> DADKLPHTKVTLVAPPQVHPHEQATKSGPKVVEFTMTIEEKKMVIDDKGTTLQAMTFNGSMPGPTLVVHEGDYVQLTLVNPATNAMPHNVDFHGATGALGGAKLTNVNPGEQATLRFKADRSGTFVYHCAPEGMVPWHVVSGMSGTLMVLPRDGLKDPQGKPLHYDRAYTIGEFDLYIPKGPDGKYKDYATLAESYGDTVQVMRTLTPSHIVFNGKVGALTGANALTAKVGETVLLIHSQANRDTRPHLIGGHGDWVWETGKFANPPQRDLETWFIRGGSAGAALYTFKQPGVYAYLNHNLIEACELGAAGHIKVEGKWND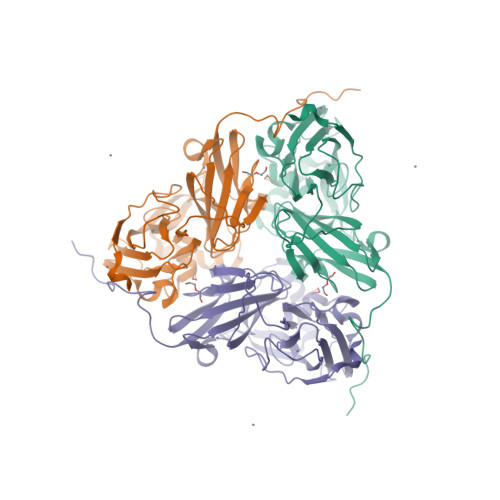DLMKQIKAPAPIPR> GPTYVQALFDFDPQEDG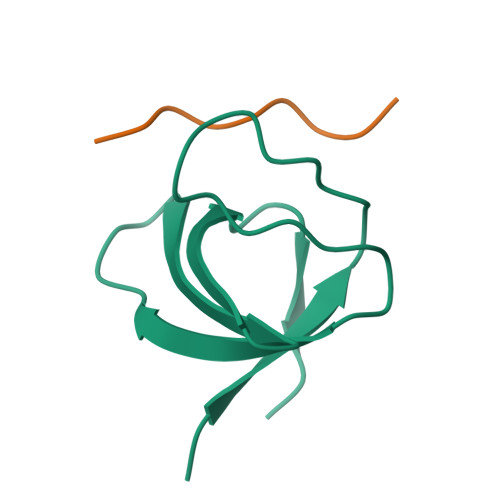ELGFRRGDFIHVMDNSDPNWWKGACHGQTGMFPRNYVTAVN;> APPPRPPKP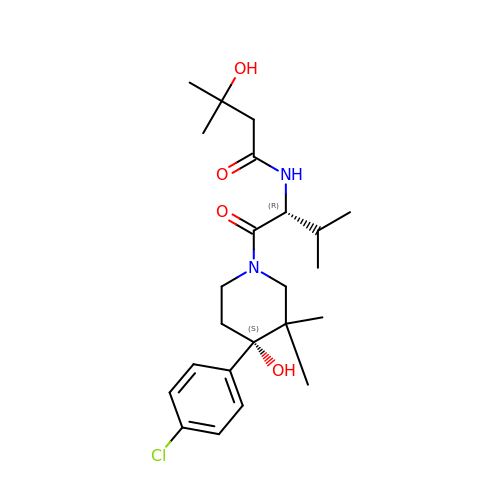N-{(2R)-1-[(4S)-4-(4-chlorophenyl)-4-hydroxy-3,3-dimethylpiperidin-1-yl]-3-methyl-1-oxobutan-2-yl}-3-hydroxy-3-methylbutanamide | C23 H35 Cl N2 O4 | PTNKPLPRPJERNR-XXBNENTESA-N>PNFAGTWKMRSSENFDELLKALGVNAMLRKVAVAAASKPHVEIRQDGDQFYIKTSTTVRTTEINFKVGEGFEEETVDGRKCRSLPTWENENKIHCTQT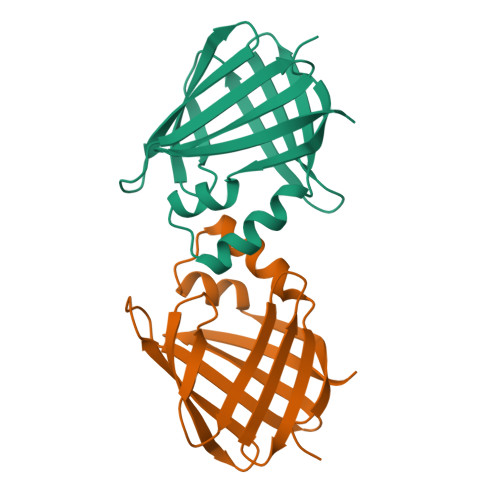LLEGDGPKTYWTRELANDELILTFGADDVVCTRIYVRE[2x]2-chloranyl-6-(4,6-dimethoxypyrimidin-2-yl)sulfanyl-benzoic 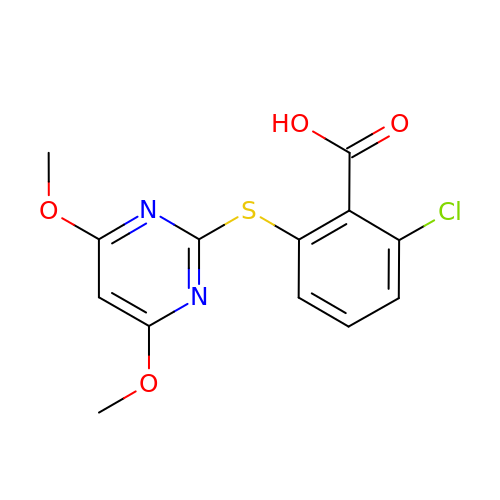acid | C13 H11 Cl N2 O4 S | QEGVVEOAVNHRAA-UHFFFAOYSA-N>[4x]SDEEEKVRFYLEQAEIHYRLGDPEAAERAIYLAKMIAAENSDPELFEEIEE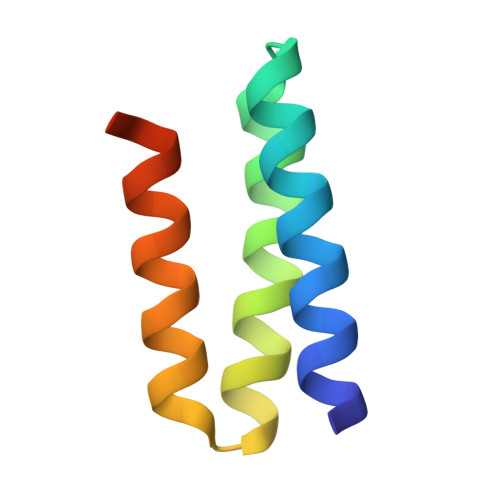FEKELLEHHHHHH>[2x]GPLGSMSDENKSTPIVKASDITDKLKEDILTISKDAL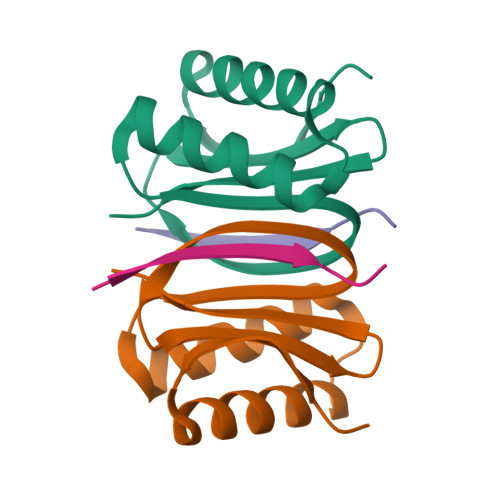DKYQLERDIAGTVKKQLDVKYGNTWHVIVGKNFGSYVTHEKGHFVYFYIGPLAFLVFKTA;>NYAESGIQTDL[2x]> MHHHHHHSENTFIFPATFMWGTSTSSYQIEGGTDEGGRTPSIWDTFCQIPGKVIGGDCGDVACDHFHHFKEDVQLMKQLGFLHYRFSVAWPRIMPAAGIINEEGLLFYEHLLDEIELAGLIPMLTLYHWDLPQWIEDEGGWTQRETIQHFKTYASVIMDRFGERINWWNTINEPYCASILGYGTGEHAPGHENWREAFTAAHHILMCHGIASNLHKEKGLTGKIGITLNMEHVDAASERPEDVAAAIRRDGFINRWFAEPLFNGKYPEDMVEWYGTYLNGLDFVQPGDMELIQQPGDFLGINYYTRSIIRSTNDASLLQVEQVHMEEPVTDMGWE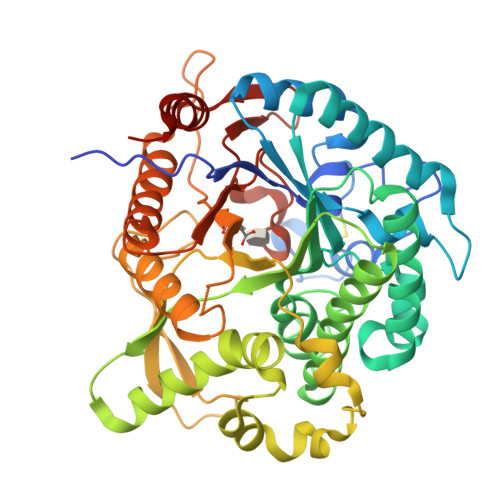IHPESFYKLLTRIEKDFSKGLPILITENGAAMRDELVNGQIEDTGRHGYIEEHLKACHRFIEEGGQLKGYFVWSFLDNFEWAWGYSKRFGIVHINYETQERTPKQSALWFKQMMAKNGF>[5x]SMEIKQSPDEFCHSDFEDASQGSDTRICPPSSLLPADRKWGFITVGYRGSCTLGREGQADAKFRRVPRILVCGRISLAKEVFGETL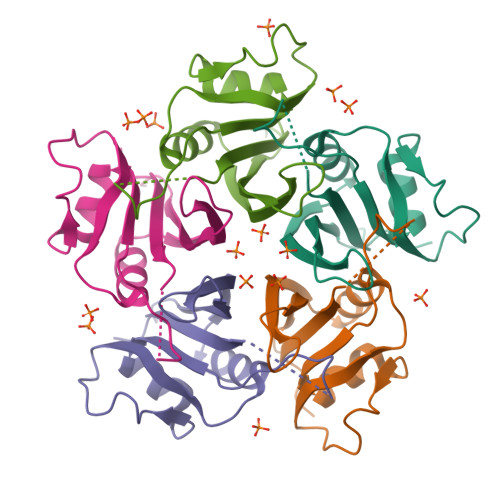NESRDPDRAPERYTSRFYLKFKHLERAFDMLSECGFHMVACNSSVTASFINQYTDDKIWSSYTEYVFYREPSRWSPS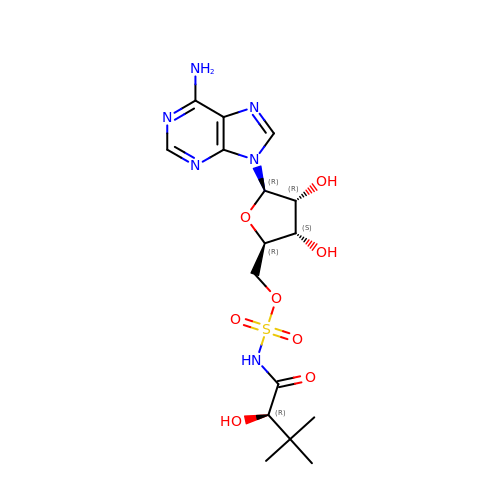5'-O-{[(2R)-2-hydroxy-3,3-dimethylbutanoyl]sulfamoyl}adenosine | C16 H24 N6 O8 S | XLQHUZMFAIRQAT-YEFHITBRSA-N>[3x]MTIDSSGYFRDAAGARFIPVGANYWPASCGVEMWQAWPEDEIFSDLDLMASLGFNTVRFFVRWPDFEPRPGEYDATMLSRLLRLLDACGERGLRPQPSLFVGWMSGGIFWPPWKSDTQNLFSDPVMIERGAAYARTITTHLKPFATHLCGIDLGNELDALPDCSAATPAQVHEWCRRMTGAIREVLPEALILSGCDHQQVIADTGWRLGGSSPCYSAGGTPAPRMVPNPAQPGIDVLTMHGYPVPNWHPVQGSGLADPLTRSLLPFYVKCARAFGPVLLQEFGTILTSRAAAPHTDAYLRAILPACREAGANGYLWWCFKDIPAPLHPYIKNNFESELGLVDIEGRVK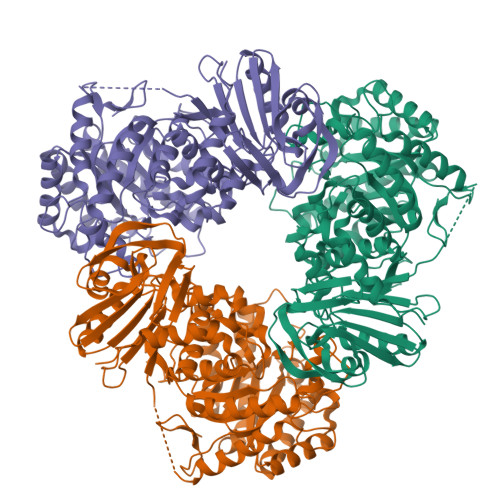KGLEYFVEFARAETQRALKVLTACEQLDHSAEDAPTVHLYWPRHYYHRNNHRNPGNEPRETSRRLILAHHLLQSAEEHVGIVRGDQPLPSPSEVERIIITGVFTGLDEIKELHSWVEQGGQLLWHAPDPVNWAQAMSRLVGAEIADYRAATPAITATDEGPYEFTCFLRGMRVRIEPRGAQILMTDNEGSPLVLRHRVGAGCVTSVLADVEASFLSQWPDRQTQEASWSAWYAALLTKDQSEGVARAHHHHHH> GGNRTFSYTLEDHTKQAFGIMNELRLSQQLCDVTLQVKYQDAPAAQFMAHKVVL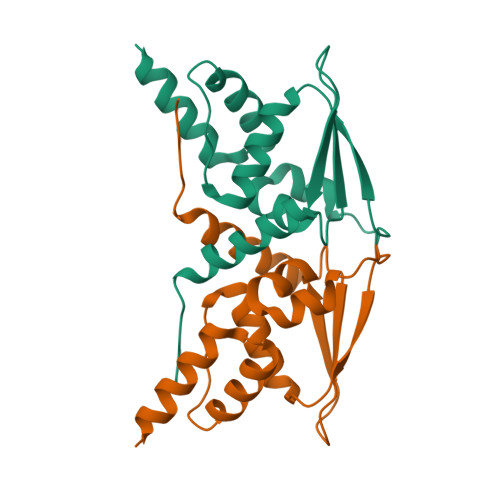ASSSPVFKAMFTNGLREQGMEVVSIEGIHPKVMERLIEFAYTASISMGEKCVLHVMNGAVMYQIDSVVRACADFLVQQLD>[24x]METSKEKTITSPGPYIVRLLNSSLNGCEFPLLTGRTLFVVGQSDALTASGQLPDIPADSFFIPLDHGGVNFEIQVDTDATEIILHELKEGNSESRSVQLNTPIQVGELLILIRPESEPWVPEQPEKLETSAKKNEPRFKNGIVAALAGFFILGIGTVGTLWILNSPQRQAAELDSLLGQEKERFQVLPGRDKMLYVAAQNERDTLWARQVLARGDYDKNARVINENEENKRISIWLDTYYPQLAYYRIHFDEPRKPVFWLSRQRNTMSKKELEVLSQKLRALMPYADSVNITLMDDVTAAGQA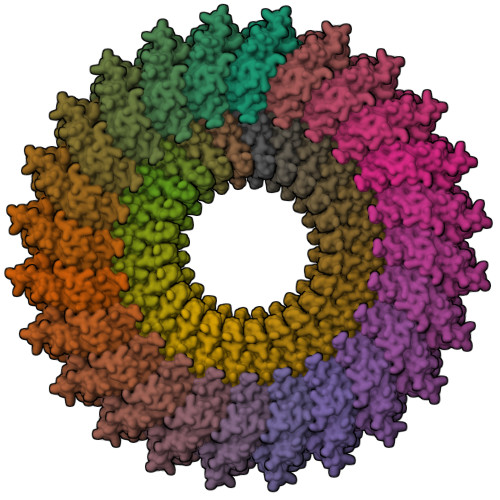EAGLKQQALPYSRRNHKGGVTFVIQGALDDVEILRARQFVDSYYRTWGGRYVQFAIELKDDWLKGRSFQYGAEGYIKMSPGHWYFPSPL;>[24x]MIRRYLYTFLLVMTLAGCKDKDLLKGLDQEQANEVIAVLQMHNIEANKIDSGKLGYSITVAEPDFTAAVYWIKTYQLPPRPRVEIAQMFPADSLVSSPRAEKARLYSAIEQRLEQSLQTMEGVLSARVHISYDIDAGENGRPPKPVHLSALAVYERGSPLAHQISDIKRFLKNSFADVDYDNISVVLSERSDAQLQAPGTPVKRNSFATSWIVLIILLSVMSAGFGVWYYKNHYARNKKGITADDKAKSSNE> GEFKPSACRNLFGPV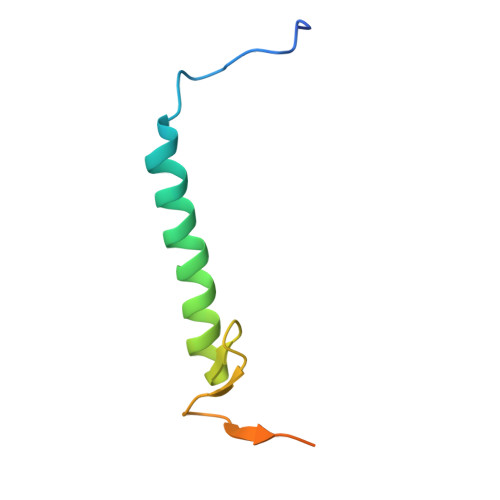DHEELTRDLEKHCRDMEEASQRKWNFDFQNHKPLEGKEEWQEVEKGSLPEFEERPPR> GSKDYDELLKYYELHETIGTGGFAKVKLACHILTGEMVAIKIMDKNTLGSDLPRIKTEIEALKNLRHQHICQLYHVLETANKIFMVLEYCPGGELFDYIISQDRLSEEETRVVFRQIVSAVAYVHS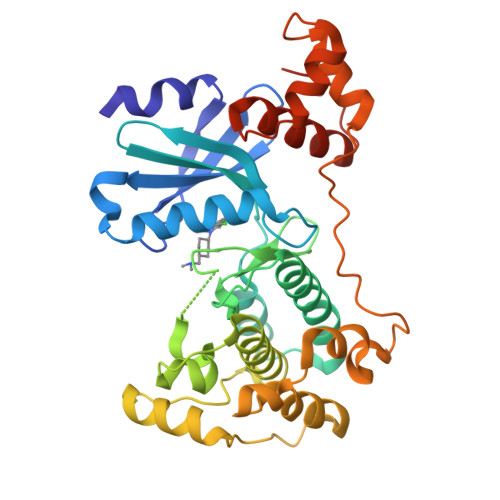QGYAHRDLKPENLLFDEYHKLKLIDFGLCAKPKGNKDYHLQTCCGSLAYAAPELIQGKSYLGSEADVWSMGILLYVLMCGFLPFDDDNVMALYKKIMRGKYDVPKWLSPSSILLLQQMLQVDPKKRISMKNLLNHPWIMQDYNYPVEWQSKNPFIHLDDDCVTELSVHHRNNRQTMEDLISLWQYDHLTATYLLLLAKKARGKPVRLRLSSFSCG Rv1411c encodes the mycobacterial lipoprotein LprG, which can bind triacylated phospholipids such as phosphatidylinositol mannoside (PIM) and lipoarabinomannan (LAM) and is necessary for normal surface display of LAM. However, unlike other known mycobacterial lipoproteins, LprG is in an operon with a putative integral membrane transporter, Rv1410, a member of the major facilitator superfamily (MFS). LprG binds TAG within a large hydrophobic cleft and is sufficient to transfer TAG from donor to acceptor membranes. Thus, we identify LprG as a physiologically important TAG transporter.

Previous work on the structure of LprG revealed a large central cavity that can accommodate triacylated lipid species, including triacylated phosphatidylinositol (Ac1PIM2). Briefly, the alpha-beta fold is maintained and consists of 10 anti-parallel ß-strands apposed by 6 α-helices that define a central cavity whose entrance is lined by multiple loops. The TAG glyceryl group is located at this entrance between loops L1 (aa 65–72) and L2 (aa 95–98). Compared to the position of Ac1PIM2 bound to LprG, the orientation of TAG is conserved: the hydrophilic glyceryl headgroup interacts with Ser72 at the cavity entrance. The acyl chains form interactions with the side chains of hydrophobic residues within the cavity. However, while the three acyl chains of Ac1PIM2 are all bound within the cavity, only two of the TAG palmitoyl chains (sn1 and sn2) are similarly buried; the third acyl chain (sn3) is exposed to the solvent. The first ten carbons of the sn3 palmitoyl chain form van der Waals contacts with the hydrophobic sidechains at the cavity entrance, including Leu95, Leu115, Phe123 and Ile129. The lid of the cavity, composed of a helix-loop motif (α2-loop1- α3-loop2), is flexible and was found in two conformations that define distinct cavity volumes. The volume of the open form with TAG bound is 1425 Å3 and the closed form is 895 Å3 due to a major inward movement of the cavity lid (aa 129–134). Comparing the helix-loop motif in the closed and open forms, the side chain of Tyr130 blocks the binding site for the sn2-palmitoyl chain of TAG.

>MHHHHHHGPLPDAKPLVEEATAQTKALKSAHMVLTVNGKIPGLSLKTLSGDLTTNPTAATGNVKLTLGGSDIDADFVVFDGILYATLTPNQWSDFGPAADIYDPAQVLNPDTGLANVLANFADAKAEGRDTINGQNTIRISGKVSAQAVNQIAPPFNATQPVPATVWIQETGDHQLAQAQLDRGSGNSVQMTLSKWGEKVQVT[2x]> IIGGDECNINEHRFLVALYTSRSRTLFCGGTLINQEWVLTAAHCDRKNFRIKLGMHSKKVPNEDEQTRVPKEKFFCLSSKNYTLWDKDIMLIRLDSPVKNSKHIAPFSLPSSPPSVGSVCRIMGWGRISPTEGTYPDVPHCVNINLLEYEMCRAPYPEFELPATSRTLCAGILEGGKDTCKGDSGGPLICNGQFQGIASWGDDPCAQPHKPAAYTKVF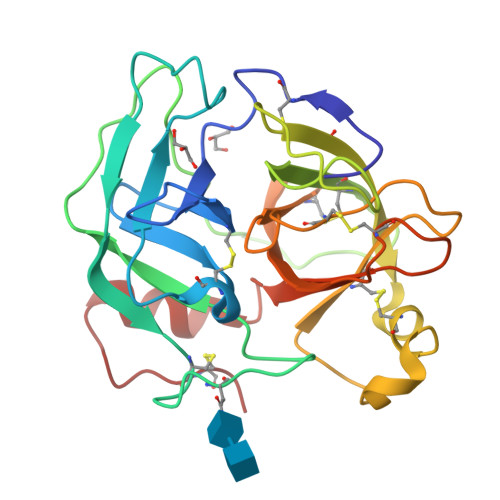DHLDWIENIIAGNTDASCPP> PLSIVRSIYNNEFQW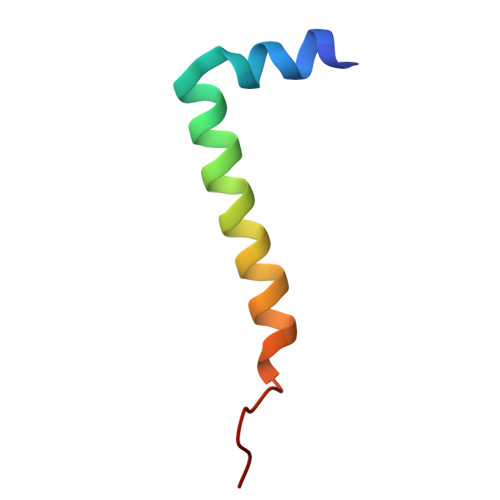MLVKSYGLFFLGVRLAKEFVGVELMPS> MARIREVQGDITE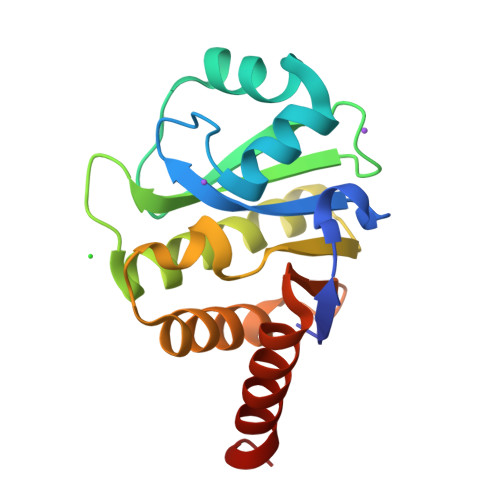FQGDAIVNAANNYLKLGAGVAGAILRKGGPSIQEECDRIGKIRVGEAAVTGAGNLPVRYVIHAAVLGDEPASLETVRKATKSALEKAVELGLKTVAFTALGAWVGGLPAEAVLRVMLEEIKKAPDTLEVTGVHGTEKSAEAARRALLEHHHHHH> GSHMEKVPGEMEIERRERSEELSEAERKAVQAMWARLYANCEDVGVAILVRFFVNFPSAKQYFSQFKHMEDPLEMERSPQLRKHACRVMGALNTVVENLHDPDKVSSVLALVGKAHALKHKVEPVYFKILSGVILEVVAEEFASDFPPETQRAWAKLRGLIYSHVTAAYKEVGWVQQVPNATTPPATLPSS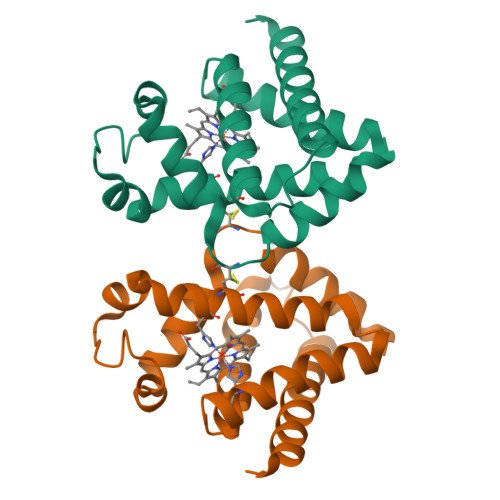GP> RVLNNLKLRELLLPKFTSLWEIQTEVTVDNRTILLTWMHLLCESFELDKSVFPLSVSILDRYLCKKQGTKKTLQKIGAACVLIGSKIRTVKPMTVSKLTYLSCDCFTNLELINQEKDILEALKWDTEAVLA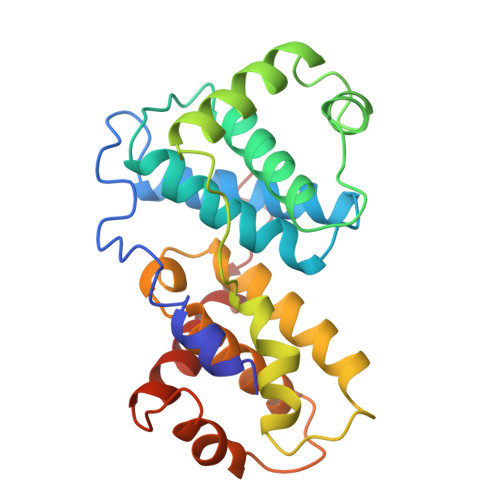TDFLIPLCNALKIPEDLWPQLYEAASTTICKALIQPNIALLSPGLICAGGLLTTIETDNTNCRPWTCYLEDLSSILNFSTNTVRTVKDQVSEAFSLYD(3E)-3-(hydroxyimino)propanoic acid | C3 H5 N O3 | 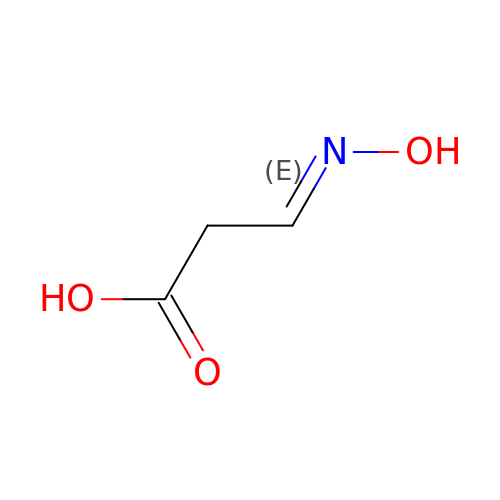XTKKYEXSKPSWOJ-DUXPYHPUSA-N> QTMCSQYDSASSPPYSVNQNLWGEYQGTGSQCVYVDKLSSSGASWHTEWTWSGGEGTVKSYSNSGVTFNKKLVSDVSSIPTSVEWKQDNTNVNADVAYDLFTAANVDHATSSGDYELMIWLARYGNIQPIGKQIATATVGGKSWEVWYGSTTQAGAEQRTYSFVSESPINSYSGDINAFFSYLTQNQGFPASSQYLINLQFGTEAFTGGPATFTVDNWTAS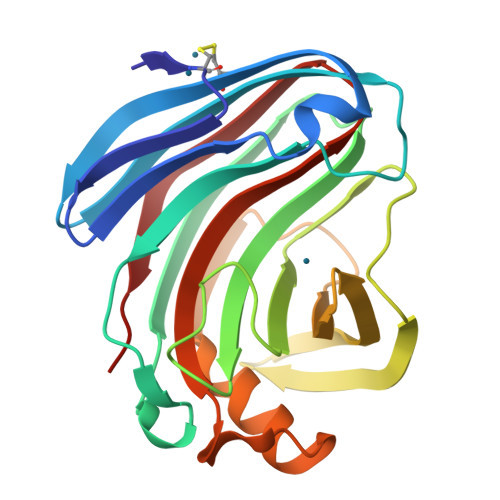VN Leucine aminopeptidase (LAP) is found in all kingdoms of life and catalyzes the metal-dependent hydrolysis of the N-terminal amino acid residue of peptide or amino acyl substrates. We report here the X-ray structures of three kinetoplastid acidic LAPs (LAP-As from Trypanosoma brucei, Trypanosoma cruzi, and Leishmania major) which were solved in the metal-free and unliganded forms, as well as in a number of ligand complexes, providing insight into ligand binding, metal ion requirements, and oligomeric state. LAPs of the M17 family of aminopeptidases are bilobal proteins with a highly conserved C-terminal domain harboring the aminopeptidase activity. They form homohexamers of approximately 330 kDa with the active sites facing a central cavity separated from the bulk solvent but accessible through solvent channels.

For both the TbLAP-A and LmLAP-A complexes, the electron density was sufficient to model the ligand, albeit with less than 100% occupancy. The TbLAP-A--actinonin complex had six molecules in the asymmetric unit, and local noncrystallography symmetry was imposed for the protein chains. The electron density for the ligand was generally poor but sufficient to build the actinonin in all six chains. Their densities varied slightly, so that the ligand was modeled in each chain individually, with variation in their conformations. Nevertheless, the actinonin coordination was identical in all chains and differed only slightly from that in LmLAP-A. Actinonin in LmLAP-A and TbLAP-A is coordinated by the Mn2+ ions and hydrogen bonds. In both structures, the two Mn2+ atoms coordinate the O-2 and O-4 oxygen atoms of the ligand. In LmLAP-A, the side chains of K299, D304, K311, and D389 form hydrogen bonds with O-2 and O-4, and the main-chain oxygen of L420 and the main-chain nitrogen of G422 form hydrogen bonds with N-1 and O-13, respectively. The corresponding residues in TbLAP-A are K289, D294, K301, D371, L402, and G404, and A405 forms an additional hydrogen bond with O-27 in four of the six chains. Superposition of the active sites including the actinonin molecules reveals the high similarity of the conformations actinonin adopts, with the only difference being in the hydroxymethyl-pyrrolidine moiety, which forms a hydrogen bond in TbLAP-A but not in LmLAP-A, where it is bent away from the corresponding residue (A424).

>[6x]MPTLPKAEAKELSAFVQSCVEYKTNVCFTDVAAYESNQKGVLSSGLAVLVGTHKQLRDPAVQRLPFYNPAVAEAIERVKEGGTYGVLVEGLANAAGSKFVRVVVGEVPTKASRNNCPARPDVVTXLVTAALDEVKEPNTTVDVFVLSNAVLPIAAAVARCGKHNFSAKDGAAAAAYNSGKVSRLQVVFPEPPAIPPKDLEAVATSTQLCQRLVDAPPNLLTTATFTEIAQGYAKALGFDVDVICGDDLCERGYGGIYSVGKAAFEAPRLVTLLYTPKGTPVKKVSLVGKGIVYDCGGLALKPADYMKLMKHDMGGAAAVFCGFLTAVRLQQPVQLSCTLCLAENAIGPKSYRNDDIIVMKSGKTVEVINTDAEGRIVLGDGVFHATNELSFTPDVVIDMATLTGAQGIATGRHHAGLYVNEEGAEAAMLRAGRESGETCFPVLYCPEYHEPEFKSNHADMTNLMERRDNAGVSCAGYFITTHLSPKFTGAHIHVDLAYPVFNSNGATGFGPALLTEYFRKL>[2x]MDTFVLDTSVFTNPDVYHQFEEDQLGAIENFISLASHTNANFFMPTSVYYEFTKMVSLGDLAPKFELVVRIRSPRKWGLMVPAEFLYEFIEEVRYRINKGLRIAEEHTKEAGKLAEEEVGRVVNRLREKYREALRAGIIDSKEDVDVLLLSYELDAILVSGDEGLRKWADRVGIKLIDPKNLRYIMENLTKVGR

One of the first steps of tRNA processing in nearly every organism is the removal of the 5′ leader sequence by ribonuclease P (RNase P). In contrast to other RNase Ps, HARPs consist only of a metallonuclease domain and lack the canonical substrate recognition domain essential in other classes of proteinaceous RNase P. We determined the cryo-EM structure of Aquifex aeolicus HARP (Aq880) and two crystal structures of Hydrogenobacter thermophilus HARP (Hth1307) to reveal that both enzymes form large ring-like assemblies: a dodecamer in Aq880 and a tetradecamer in Hth1307. HARP structures in additional oligomeric states have also been published, including HARP dimers from Planctomyces bacterium and Thermococcus celer and a HARP tetramer from P. bacterium complexed with Escherichia coli pre-tRNAHis. These data all show that a monomer of HARP is a VapC-like endonuclease that consists of a PIN domain-like metallonuclease domain and two protruding α helices, which are thought to be responsible for substrate recognition. The active site is conserved among HARPs and PRORPs, with five negatively charged residues, predominantly aspartate, positioned to coordinate two catalytic magnesium ions.

We sought to better understand the structure and function of Hth1307 using protein crystallography. From the lower molecular weight fraction of Hth1307 discussed above, we first determined the crystal structure of Hth1307 to 2.5 Å as a dimer within the asymmetric unit. The homotetrameric Hth1307 assembly is generated through symmetry by two identical dimers resulting in a dimer of dimers. Each monomer in the Hth1307 dimer consists of a PIN-like metallonuclease domain and a spike helix (SH) domain. The SH domain is a protruding α-helical domain consisting of helices α6 and α7, which substantially contribute to the dimerization interface by forming an extensive four-helical bundle. In the tetramer, two dimers come together in a side-by-side arrangement, where the two dimers are angled at 41°. The tetramer interface is considerably smaller than the dimer interface, with a surface area of 589.5 Å2 between monomers, for a total of 1179.0 Å2 across the entire interface. The 5′ end of the acceptor stem is positioned in the metal active site, and the T and D loops are recognized by the pentatricopeptide repeat domain in PRORP and MRPP3 (32) and the CR-II/CR-III modules in human and bacterial RNP RNase P. This arrangement allows RNase Ps to recognize tRNA structural elements and select substrates through a molecular ruler mechanism. Upon inspection of the electrostatic surface of the tetramer, there is a positively charged region of the SH domain (Fig. S7, (38)) that includes residues R125, R127, K129, and R131, which have been confirmed to be necessary for pre-tRNA processing activity.> SGRGXGGXG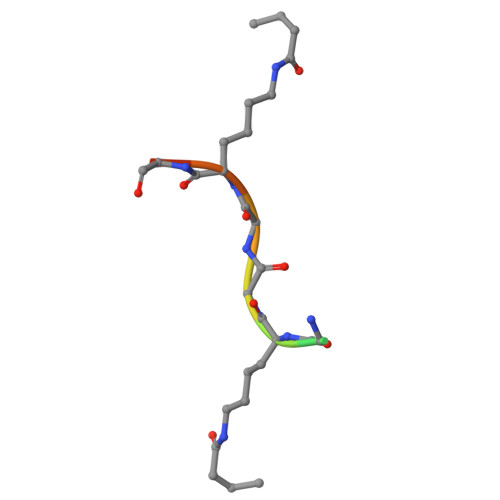LG>[2x]MRIVRRRPAATLLRHLALVAAALPVLAGTASAAPPTDRYAAPGLEKPASILIDRWGVPHIYAGTLYDAFYAQGFIAARDRLWQIDLWRKRGLGEMARDFGPAYVDGDRMARAVLYRGDMYREWLAYGSDAKRVAEAFVAGVNAYVALTEAQPELLPREFKQLGYKPSRWRAEDIVRIRHHGETLNFTGEVDRATLYCQ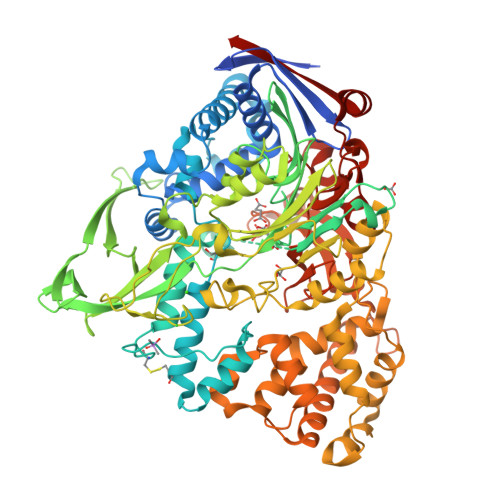AKEQAARADWLRRELDPPITPTLPEGLDPCAVPAAALKKAYTLATAAANFPKEAWQKASADAVPVDQLYAAVDANSDTGRSLGSNNWVIAGSRTSTGRPILANDPHRAHGAPSLRYVSHLNAPGLSVIGAGEPFLPGISIGHNGTIAFGLTRFYMDQEDLYVYETDPAQPKSYRYRGRWEPMETITEKITVRGEAEPRTVTIDFTRHGPVLHADDASHRAWALRAAWLDTGMAPYFGSMDYMRATNWDQFRAAMNRWGAPGENQVYADRNGNIGWIPGGLTVIRPNWDGLFPVPGDGRYEWAGYRNMDELPWAYNPSTGHIVTANENNIPPDHPAAKLGVGYEWSDSSRARRLKSLVAAAPVSSLRDSIAWQNDTVSLPAQRTLAVMRTVGNAGAAASLLQDPQVQRAVALLRGWDGNVRADSVPAALFEIWFSNHLRQAVVRAALPEDAAKLVGAGDAARVLAVLEQPDTWMPTARRDEVMLTSLKAAMAELERRSPSPEKLATWGTLHRAIFRHPLANIVDDATRAQYNVDAGGIGGSAFTPMNTSYRNSDYHLTAGASFRMVLDVGNWDQGRVVNTPGQSGDPGNSHYRDLAPIWAKGQTFPLVYSRKAVERAAEKRIELTPR>[4x]MNRVVGFIGLGRMGQAICRRLLASQMPVHVHNRSREKADDLIRQGAVWAPDIVALTRAARVLFVCTAGSEAVQDFYHAPDRGLLACLEVGDIVVDLSTIAPETAEGLHAAFAQQGADYIECPVSGGVEGA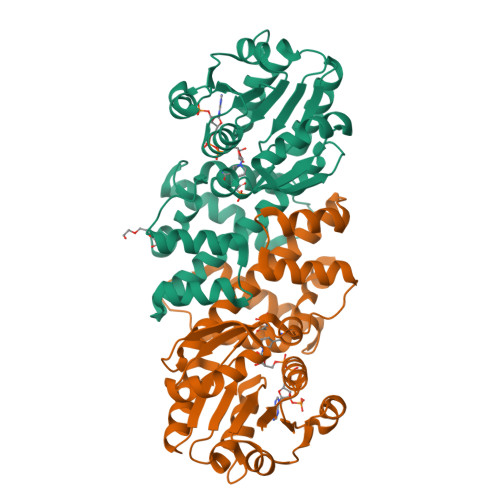LAGILSAIVSGRPEAYGLIRPLLEVFCATVTYVPEPGKAQRLKILNNLAESINLAGAIEVISQGLSQGLDLKSMADVFTSCRGRSAYMDVALGYALSGGASSNVSLGVRCKDLELARRRLPQDQSYPFSTLAMTTFDTVRQACGEESDQCQYFSVLSHNKAWKAS> ADLVPPPGYYAAVGERKGSAGSCPAVPPPYTGSLVFTSKYEGSDSARATLNVKAEKTFRSQIKDITDMERGATKLVTQYMRSGRDGDLACALNWMSAWARAGALQSDDFNHTGKSMRKWALGSLSGAYMRLKFSSSRPLAAHAEQSREIEDWFARLGTQVVRDWSGLPLKKINNHSYWAAWSVMSTAVVTNRRDLFDWAVSEFKVAANQVDEQGFLPNELKRRQRALAYHNYALPPLAMIAAFAQVNGVDLRQENHGALQRLAERVMKGVDDEETFEEKTGEDQDMTDLKVDNKYAWLEPYCALYRCEPKMLEAKKDREPFNSFRLGGEVTRVFS

The alg operon also encodes a periplasmic lyase, AlgL. Characterization of this enzyme in vitro demonstrated that it preferentially degrades nonacetylated polymannuronate (polyM) via a ß-elimination mechanism. The structure reveals that AlgL adopts an (α/α)5 toroid fold with five pairs of antiparallel α-helices. Our in vivo studies demonstrate that AlgL does not associate with other alginate biosynthetic proteins and functions as a periplasmic homeostasis enzyme to clear the periplasm of accumulated alginate to prevent cell lysis.

To enable our functional in vivo studies of AlgL and delineate the role of this enzyme in alginate biosynthesis, we first determined its structure, minus its signal sequence (NHis6-AlgL28–362), to 1.65 Å resolution using selenomethionine (SeMet) incorporation and the single-wavelength anomalous dispersion (SAD) technique. AlgL crystallized in space group P212121 with one molecule in the asymmetric unit. Although we cocrystallized the protein with a mannuronate trisaccharide (ManA3), we were only able to detect electron density for a sugar monomer suggesting perhaps that cleavage of the ManA3 substrate may have occurred in crystallo or that the remaining sugar units/moieties were disordered in the structure. While this ManA identifies the location of the active site, we anticipate that it will contain multiple sugar-binding sites given that AlgL’s activity increases linearly with the number of residues in the substrate. Indeed, examination of the enzyme’s surface electrostatic properties and residue conservation revealed an elongated, highly conserved, and strongly electropositive groove. In addition to the pronounced, long substrate-binding groove, we also identified an extended loop that partially closes over the ManA-binding site, known as the lid-loop. Similar to Y246F A1-III, the sugar monomer modeled in our AlgL structure occupies subsite +1. However, this monomer adopts a different orientation; a variation that is most likely attributable to the lack of additional conformational restraints that a longer sugar polymer would provide. The conformation of the lid-loop correlates with the presence of a ligand in the +1 subsite, with the lid-loop in the Y246F A1-III and AlgL structures in a more enclosed conformation, while the loop adopts a more open conformation in the WT A1-III structure. In our AlgL structure, we found that the Nζ atom of lid-loop residue K66 interacts via a hydrogen bond with the hydroxyl group of the C-2 of ManA.>MTIEYATRHRARSFIPPEPGKPYFIEKGLGDRAHLFGDLITIYAGGEQTENTFNFFTCEGPKGEVIPAHSHADTYEVFYITQGAVRLFVEDLEGEQHEKLLTPGDFGFVPKNCVHAYRMERHHSQVVGVAAGPGGTFERFFESLGTPAEELGLPVRPFVPEPEKFR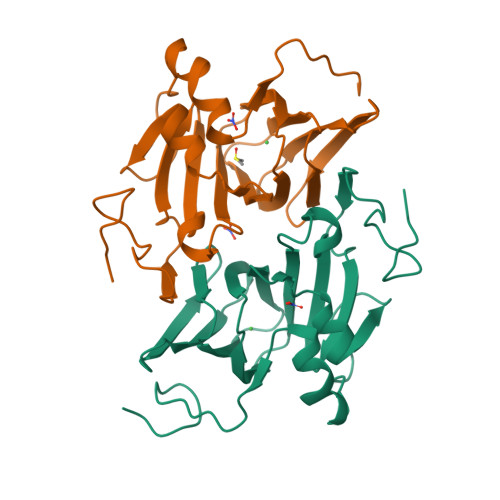TVPEQYDVRFRPDHQWHTGSIEGRKL[2x]>IQTTAPPVKESSFVEKMKKTGRNIIVFYGSQTGTAEEFANRLSKDAHRYGMRGMSADPEEYDLADLSSLPEIDKSLVVFCMATYGEDPTDNAQDFYDWLQETDVDLTGVKFAVFGLGNKTYEHFNAMGKYVDQRLEQLGAQRIFELGLGDDDGNLEEDFITWREQFWPAVCEFFGVEATGEESSIRQYELVVHEDMDVAKVYTGEMGRLKSYENQKPPFDAKNPFLAAVTANRKLNQGTERHLMHLELDISDSKIRYESGDHVAVYPANDSALVNQIGEILGADLDVIMSLNNLDEESNKKHPFPCPTTYRTALTYYLDITNPPRTNVLYELAQYASEPSEQEHLHKMASSSGEGKELYLSWVVEARRHILAILQDYPSLRPPIDHLCELLPRLQARYYSIASSSKVHPNSVHICAVAVEYEAKSGRVNKGVATSWLRAKEPAGENGGRALVPMFVRKSQFRLPFKSTTPVIMVGPGTGIAPFMGFIQERAWLREQGKEVGETLLYYGCRRSDEDYLYREELARFHKDGALTQLNVAFSREQAHKVYVQHLLKRDREHLWKLIHEGGAHIYVCGDARNMAKDVQNT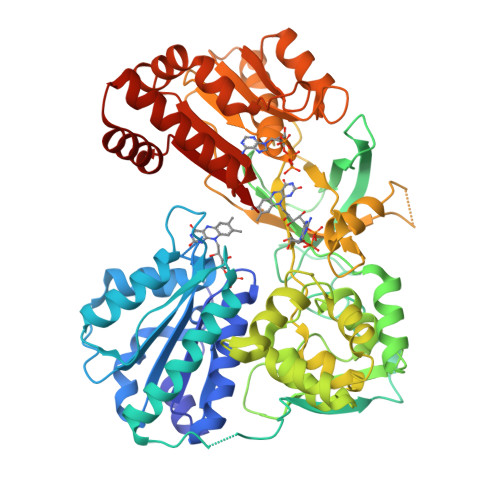FYDIVAEFGPMEHTQAVDYVKKLMTKGRYSLDVWS[2x]The colE proteins are nonspecific DNases, which are produced by Escherichia coli to eliminate neighboring bacteria. To avoid autotoxicity, the producing cells co-express Im proteins, which tightly bind and inhibit colE’s activity. In the colE/Im system, comprising four homologous pairs (colEwt2/Imwt2, colEwt7/Imwt7, colEwt8/Imwt8, and colEwt9/Imwt9), each cognate pair forms an ultrahigh affinity complex (KD < 10−13 M), whereas the non-cognate pairs show non-protective affinities (KD > 10−10 M). Our results demonstrate that the design of substantially different backbone conformations, orientations, and sequences at the binding site generates dozens of new interaction pairs from a single starting one.

To verify the atomic accuracy of the design procedure, we determined the structures of two designed pairs by X-ray crystallography: colEdes3/Imdes3 with >3 orders of magnitude pairwise specificity relative to the wild-type colEwt2/Imwt2 and colEdes7/Imdes7 with low Im specificity. In both structures, the conserved hotspot region formed as predicted. To test whether cognate affinity could be improved, we focused on colEdes3/Imdes3, which exhibited KD = 73 nM and at least three orders of magnitude pairwise specificity relative to colEwt2/Imwt2. Furthermore, the high-specificity design, colEdes3/Imdes3 showed high accuracy throughout loop I (0.5 Å Cα rmsd over all Im side chains). The designed rigid-body orientation and side-chain conformations at the interface were also atomically accurate, except two polar side chains (Asn31 and Gln34) that reoriented due to a water molecule that was not modeled by Rosetta. Apart from this difference, the polar interaction network in this complex formed with remarkably high accuracy compared to the designed one. Due to backbone preorganization, the designed polar interactions can only form accurately in the cognate pairs as seen in the crystallographic analysis of the high-specificity pair colEdes3/Imdes3.

>MESKRNKPGKATGKGKPVGDKWLDDAGKDSGAPIPDRIADKLRDKEFKNFDDFRKKFWKEVAKDPDLAKQFSKANQRNIKDGNAPFARESDQVGGRTTYELHHDKPISQDGGVYDMNNIRVTTPKRAIDIHRGK[2x];>[2x]MELKHSISDYTEAEFLEFVKDIFRLSRPQDNDLQIKLVLEFKRLTEHPDGSDLIYYPRSDREDSPEGIVKEIKEWRAANGKSGFKQGLEHHHHHH> INITSSASQEGTRLNLICTVWHKKEEAEGFVVFLCKDRS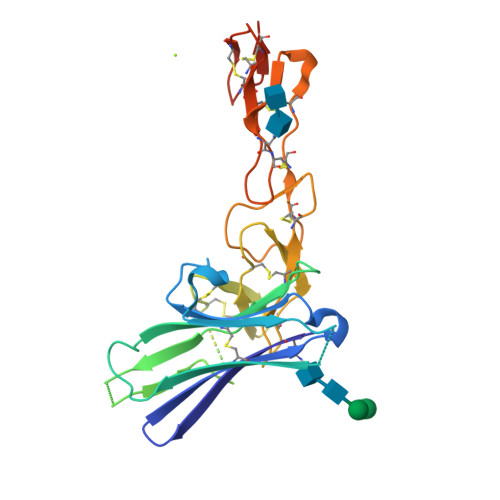GDCSPETSLKQLRLKRDPGIDGVGEISSQLMFTISQVTPLHSGTYQCCARSQKSGIRLQGHFFSILFTETGNYTVTGLKGGGGSGGGGSGGGGSGGGGSLPSCKEDEYPVGSECCPKCSPGYRVKEACGELTGTVCEPCPPGTYIAHLNGLSKCLQCQMCDPAMGLRASRNCSRTENAVCGCSPGHFCIVQDGDHCAACRAYATGHHHHHH> DHQVKDSLEQLRCHFTWELSIDDDEMPDLENRVLDQIEFLDTKYSVGIHNLLAYVKHLKGQNEEALKSLKEAENLMQEEHDNQANVRSLVTWGNFAWMYYHMGRLAEAQTYLDKVENICKKLSNPFRYRMECPEIDCEEGWALLKCGGKNYERAKACFEKVLEVDPENPESSAGYAISAYRLDGFKLATKNHKPFSLLPLRQAVRLNPDNGYIKVLLAL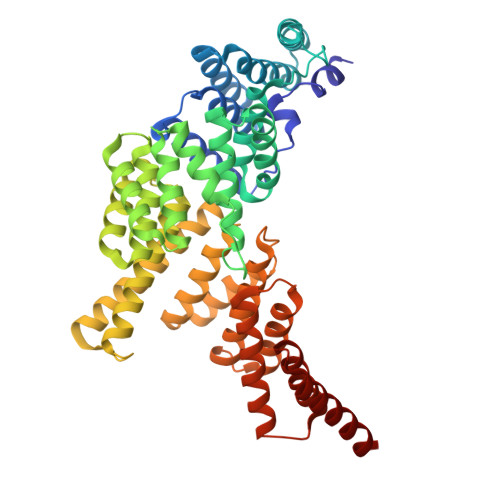KLQDEGQEAEGEKYIEEALANMSSQTYVFRYAAKFYRRKGSVDKALELLKKALQETPTSVLLHHQIGLCYKAQMIQIKEATKGQPRGQNREKLDKMIRSAIFHFESAVEKKPTFEVAHLDLARMYIEAGNHRKAEENFQKLLCMKPVVEETMQDIHFHYGRFQEFQKKSDVNAIIHYLKAIKIEQASLTRDKSINSLKKLVLRKLRRKALDLESLSLLGFVYKLEGNMNEALEYYERALRLAADFE>MGSDKIHHHHHHENLYFQGMKRHYIFASHGSFANGLLNSVELILGKQPDIHTLCAYVEEEVDLTQQVEALVARFPAQDELIVITDIFAGSVNNEFVRFLSRPHFHLLSGLNLPLIIDLLISAAEDNTEKLITEALTNAKESIQYCNQTIA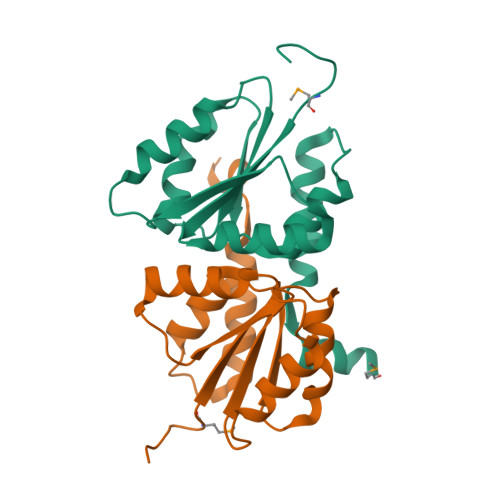SAMTMDKDF[2x]N~2~-({[(1R)-1-(4-BROMOPHENYL)ETHYL]AMINO}CARBONYL)ASPARAGINYL-N~1~-{4-{[AMINO(IMINO)METHYL]AMINO}-1-[2,3-DIHYDRO-1,3-THIAZOL-2-YL(HYDROXY)METHYL]BUTYL}VALINAMIDE | C27 H42 Br N9 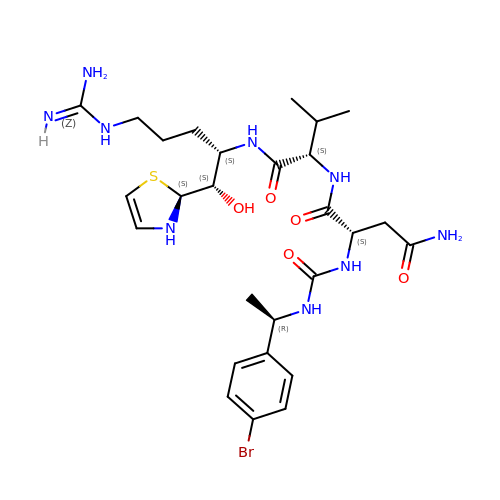O5 S | JOESWSPHHQIQBV-JJYDKGGZSA-N> MRAGLLEGVIKEKGGVPVYPSYLAGEWGGSGQEIEVKSPIDLATIAKVISPSREEVERTLDVLFKRG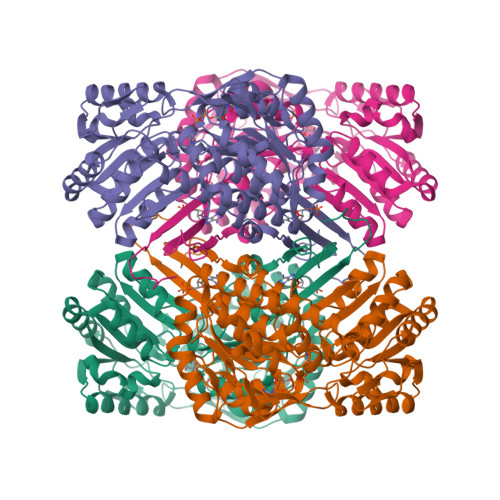RWSARDMPGTERLAVLRKAADIIERNLDVFAEVLVMNAGKPKSAAVGEVKAAVDRLRLAELDLKKIGGDYIPGDWTYDTLETEGLVRREPLGVVAAITPFNYPLFDAVNKITYSFIYGNAVVVKPSISDPLPAAMAVKALLDAGFPPDAIALLNLPGKEAEKIVADDRVAAVSFTGSTEVGERVVKVGGVKQYVMELGGGDPAIVLEDADLDLAADKIARGIYSYAGQRCDAIKLVLAERPVYGKLVEEVAKRLSSLRVGDPRDPTVDVGPLISPSAVDEMMAAIEDAVEKGGRVLAGGRRLGPTYVQPTFVEAPADRVKDMVLYKREVFAPVALAVEVKDLDQAIELANGRPYGLDAAVFGRDVVKIRRAVRLLEVGAIYINDMPRHGIGYYPFGGRKKSGVFREGIGYAVEAVTAYKTIVFNYKGKGVWKYE> MGTRDDEYDYLFKVVLIGDSGVGKSNLLSRFTRNEFNLESKSTIGVEFATRSIQVDGKTIKAQIWDTAGLERYRAITSAYYRGAVGALLVYDIAKHLTYENVERWLKELRDHADSNIVIMLVGNKSDLRHLRAVPTDEARAFAEKNGLSFIETSALDSTN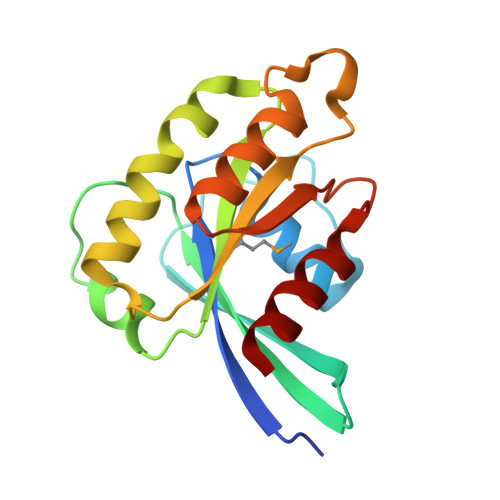VEAAFQTILTEIY>MQHNLIAFLSDVGSADEAHALCKGVMYGVAPAATIVDITHDVAPFDVREGALFLADVPHSFPAHTVICAYVYPETGTATHTIAVRNEKGQLLVGPNNGLLSFALDASPAVECHEVLSPDVMNQPVTPTWYGKDIVAACAAHLAAGTDLAAVGPRIDPKQIVRLPYASASEVEGGIRGEVVRIDRAFGNVWTNIPTHLIGSMLQDGERLEVKIEALSDT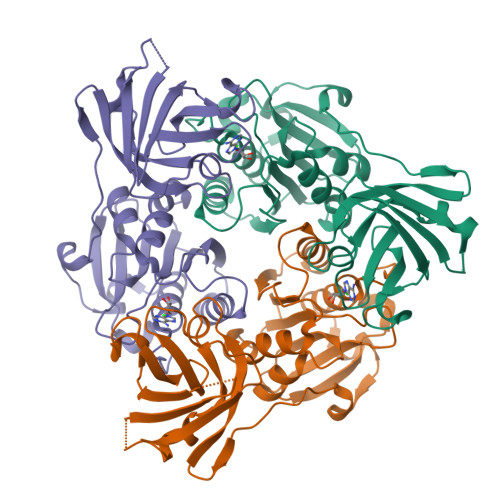VLELPFCKTFGEVDEGQPLLYLNSRGRLALGLNQSNFIEKWPVVPGDSITVSPRVPDSNLGPVLG[3x]The Dictyostelium discoideum dye-decolorizing peroxidase (DdDyP) is a newly discovered peroxidase, which belongs to a unique class of heme peroxidase family that lacks homology to the known members of plant peroxidase superfamily. DdDyP catalyzes the H2O2-dependent oxidation of a wide-spectrum of substrates ranging from polycyclic dyes to lignin biomass, holding promise for potential industrial and biotechnological applications. The overall architecture of DdDyP is similar to that of the typical DyP-type peroxidase superfamily. DdDyP contains a duplicated ferredoxin-like fold domain arranged as a β-barrel at the N- and C-terminals of the protein.

Here, we show that expressing the DdDyP peroxidase in ×2 YT enriched medium at low temperature (20°C), without adding heme supplement or biosynthetic precursors, allows for a correct native incorporation of heme into the apo-protein, giving rise to a stable protein with a strong Soret peak at 402 nm. Further, we crystallized and determined the native structure of DdDyP at a resolution of 1.95 Å, which verifies the correct heme binding and its geometry. Native DdDyP peroxidase is crystallized in a tetragonal space group P41 21 2 similar to previously reported structures, with exception that the X-ray data of the current crystal condition can be equally processed and resolved in an additional space group (P43 21 2). Moreover, the crystal unit cell exhibited significantly shorter axes, giving rise to about 35% smaller cell volume with 52.8% solvent content and 2.62 Å3 Da−1 of Matthew’s coefficient (V m), indicating the presence of a single molecule per asymmetric unit. The native structure of DdDyP accommodates heme b in a hydrophobic binding pocket flanked by the unique β-sheet at the distal side of the heme plane, the α-helices of the ferredoxin-like fold domain II and a distinct long loop at its proximal side similar to previously reported DyP structures. Our structural analysis shows that the native DdDyP heme is hexacoordinated, of which the pyrrole rings of porphyrin contributed to tetradentate chelation via their nitrogen atoms and via the conserved His222 at the proximal side with a distance of 2.11 Å. The sixth coordination is provided by a water molecule (wat-184) with a distance of 2.79 Å, which is shorter by ∼0.1 Å than that of the reported Fe(III)─CN distance, indicating a stronger coordination to Fe(III). Wat-184 forms a strong hydrogen bond (∼2.2 Å) with wat-182 and a weaker hydrogen bond with the catalytic residue Arg239. On the other hand, wat-182 interacts via strong hydrogen bonds with the second catalytic residue Asp149 as well as Ser241, suggesting that these residues may act as proton acceptors to the H2O2 during the formation of compound I oxyferryl thereby contributing to its stabilization along with Arg239 as revealed in other A-type DyP peroxidases.

> MAQSTVLPMHCLYGIFLEGNLKIQKNDQEGLKKFKDNIKKFTLELDEIDKISPQSRIGGAICFSSDIWDTVTKKISKPKELKSVNTLSSYMPGTSQRDILIHIISDRMDTCFKLAQDTMRNFGEDQLDIKQEIHGFRRVEERDLTDFIDGTENPDGDELRTQYGLVAAGQPNEFGSYVFTQRYVHNLKKWYPEPLSVQQDTVGRTKKDSIEIPRDKRPITSHVSRTDLSENGKDLKIVRQSLPYGQITGEKGLMFIAYACSLHNIEKQLQSMFGQLDGKHDLLLKYTTPVTGSFYFAPSKKELLEL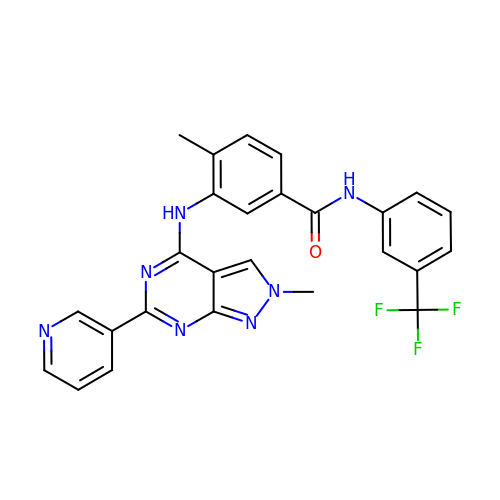4-methyl-3-[(2-methyl-6-pyridin-3-yl-pyrazolo[3,4-d]pyrimidin-4-yl)amino]-~{N}-[3-(trifluoromethyl)phenyl]benzamide | C26 H20 F3 N7 O | MWKSRKSEWLRPBL-UHFFFAOYSA-N>[2x]DPGTIVHNFSRTEPRTEPAGGSHSGSSSKLQALFAHPLYNVPEEPPLLGAEDSLLASQEALRYYRRKVARWNRRHKMYREQMNLTSLDPPLQLRLEASWVQFHLGINRHGLYSRSSPVVSKLLQDMRHFPTISADYSQDEKALLGACDCTQIVKPSGVHLKLVLRFSDFGKAMFKPMRQQRDEETPVDFFYFIDFQRHNAEIAAFHLDRILDFRRVPPTVGRIVNVTKEILEVTKNEILQSVFFVSPASNVCFFAKCPYMCKTEYAVCGKPHLLEGSLSAFLPSLNLAPRLSVPNPWIRSYTLAGKEEWEVNPLYCDTVKQIYPYNNSQRLLNVIDMAIFDFLIGNMDRHHYEMFTKFGDDGFLIHLDNARGFGRHSHDEISILSPLSQCCMIKKKTLLHLQLLAQADYRLSDVMRESLLEDQLSPVLTEPHLLALDRRLQTILRTVEGCIVAHGQQSVIVDGPVEQ;>RDPGPRRSESPPGPGGDASLLARLFEHPLYRVAVPPLTEEDVLFNVNSDTRLSPKAAENPDWPHAGAEGAEFLSPGEAAVDSYPNWLKFHIGINRYELYSRHNPAIEALLHDLSSQRITSVAMKSGGTQLKLIMTFQNYGQALFKPMKQTREQETPPDFFYFSDYERHNAEIAAFHLDRILDFRRVPPVAGRMVNMTKEIRDVTRDKKLWRTFFISPANNICFYGECSYYCSTEHALCGKPDQIEGSLAAFLPDLSLAKRKTWRNPWRRSYHKRKKAEWEVDPDYCEEVKQTPPYDSSHRILDVMDMTIFDFLMGNMDRHHYETFEKFGNETFIIHLDNGRGFGKYSHDELSILVPLQQCCRIRKSTYLRLQLLAKEEYKLSLLMAESLRGDQVAPVLYQPHLEALDRRLRVVLKAVRDCVERNGLHSVVDDDLDTEH[2x]

The Fam20 proteins are recently identified kinases that regulate essential cellular processes by phosphorylating proteins and proteoglycans. The human genome encodes three Fam20 paralogs: Fam20A, Fam20B, and Fam20C13. Remarkably, each has a distinct biochemical activity. Here, we use a combination of structural biology, biochemistry, and phylogenetics to elucidate the molecular functions and evolutionary relationships of the three Fam20 kinases.

To elucidate the molecular basis of how Fam20A regulates Fam20C activity, we determined the crystal structure of the human Fam20A−Fam20C complex. The structure reveals that Fam20A and Fam20C form a reversed face-to-face heterodimer. The Fam20A−Fam20C interface buries ~1000 Å2, or ~5% of the solvent-accessible surfaces from each molecule. At the heart of the interface are interactions between the Kβ3-Kα3 loop (we use “K” to denote the kinase core, and “N” to denote the N-terminal segment) and the N-lobe insertion domain (Kβ5-Kβ7) of each molecule. Specifically, Ile214A, Phe251A, Phe252A, Ile255A, and Leu365A form a continuous hydrophobic surface patch on Fam20A that docks onto Fam20C residues including Phe354C, Pro357C, Tyr364C, and Thr373C. Phe306A and Pro309A form hydrophobic interactions with Phe300C, and Phe306A also forms a cation−π interaction with Lys413C. In both structures, an ATP molecule (ATP-1) is bound to Fam20A in an inverted orientation, as we previously reported. In the human Fam20A−Fam20C crystal, an additional ATP (ATP-2) is bound to Fam20A perpendicularly to ATP-1, and is incompatible with tetramer formation because it would sterically occlude the Nα2 helix in Fam20C. In agreement with this observation, excess ATP converts the human Fam20A−Fam20C tetramer to a dimer in solution. The F251A/F252A and F306A/P309G mutants of Fam20A failed to activate the Fam20C Raine mutants, whereas I255E and L365D showed only partial activation. The various defects of these Fam20A mutants confirm that the dimer interface observed in the crystal structure is critical for Fam20A to bind Fam20C and regulate its activity.> GEEDKTNYGSRTVLVYIAGDNSLSRFASEDLNEMIEGMQSVDDNHNNLLVYMDKGSNPKLIRLRKDKDVVVQDVIATYDAQNSVDVDVMKNVFTTAFSHYPADSYGVVFWSHGDGWLPYNNPSTRWWGQDTGNGDNRMNIPDLNEALSVAPHFDFILFDACYMQSVEVVYQLRNRADYFIGSPTEIPGPGAPYEVVVPALFAVNSPAVSIAENYYSVYAKKYNSTGAGISNENWTGGVSISVIKSSELSALAAATRDVLQTAVSMQQSHNIDISSILCYDPLRENNYHDLMGLMQSIQGNSQAFNHYKEMYKNAVIWKNTTDNNYCTYSSGYGKMVSMDGFEGVSTYILRENNSSQEKYYRQF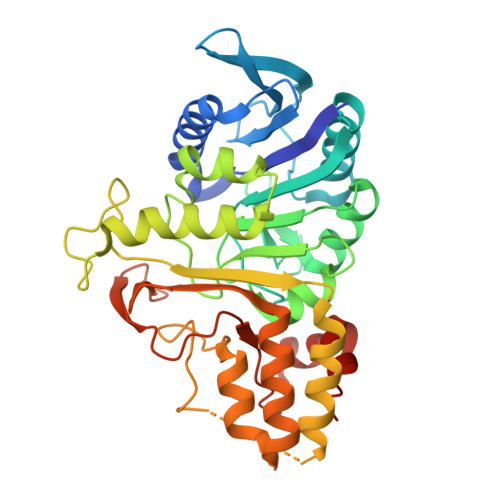VEWYSAADWDSVDW>AGFQLNEFSSSGLGRAYSGEGAIADDAGNVSRNPALITMFDRPTFSAGAVYIDPDVNISGTSPSGRSLKADNIAPTAWVPNMHFVAPINDQFGWGASITSNYGLATEFNDTYAGGSVGGTTDLETMNLNLSGAYRLNNAWSFGLGFNAVYARAKIERFAGDLGQLVAGQIMQSPAGQTQQGQALAATANGIDSNTKIAHLNGNQWGFGWNAGILYELDKNNRYALTYRSEVKIDFKGNYSSDLNRAFNNYGLPIPTATGGATQSGYLTLNLPEMWEVSGYNRVDPQWAIHYSLAYTSWSQFQQLKAT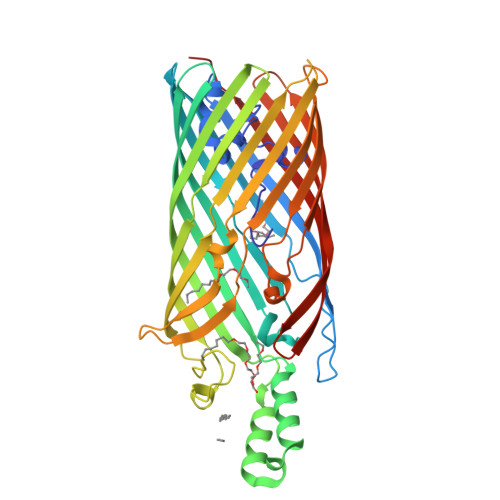STSGDTLFQKHEGFKDAYRIALGTTYYYDDNWTFRTGIAFADSPVPAQNRSISIPDQDRFWLSAGTTYAFNKDASVDVGVSYMHGQSVKINEGPYQFESEGKAWLFGTNFNYAFHHH[2x]Aminoacyl-tRNA synthetases have become the focus of drug discovery programs in several disease areas. − Compounds that target leucyl tRNA synthetase have already entered clinical development for TB treatment. This report focuses on lysyl tRNA synthetase (LysRS), the enzyme that charges lysyl tRNA with lysine. Aminoacyl-tRNA synthetases are an essential part of the protein biosynthesis machinery, responsible for charging tRNA with the appropriate cognate amino acid for incorporation into growing polypeptide chains. Molecules have been reported previously targeting LysRS in Plasmodium that block parasite growth. , LysS, the gene that encodes LysRS, is known to be essential for   − and has been classified in the top 200 most vulnerable genes to target for inhibition of growth. The crystal structures had confirmed that the compounds from this series were occupying the ATP pocket of LysRS.

Following the successful addition of a hydroxyl group at the two-position of the cyclohexyl ring, it was subsequently examined at the 3- and 4-positions with a methoxy at R2. At the 4-position, the hydroxyl retained potency against LysRS and gained KARS1 selectivity compared to 24. In KARS1, the equivalent residue is Asn497, which forms hydrogen bonds with the bound substrate lysine and Arg485, thereby blocking access to this part of the pocket. In LysRS, Thr425 is too distant from the bound substrate lysine and Lys413 (Arg485 in KARS1) to establish this hydrogen bond network, thereby allowing access of 27 and explaining the gain in selectivity. The crystal structure of 27 indicated that there was space to extend the hydroxy group deeper into the pocket. In a bid to develop this further, to explore the potential for interaction at the 4-position, a carbon spacer was added; again, this displayed good LysRS potency, but the slight decrease in MIC potency, for both 27 and 28, prevented further scope for optimization.

> MGSSHHHHHHSSGENLYFQGHMSAADTAEDLPEQFRIRRDKRARLLAQGRDPYPVAVPRTHTLAEVRAAHPDLPIDTATEDIVGVAGRVIFARNSGKLCFATLQDGDGTQLQVMISLDKVGQAALDAWKADVDLGDIVYVHGAVISSRRGELSVLADCWRIAAKSLRPLPVAHKEMSEESRVRQRYVDLIVRPEARAVARLRIAVVRAIRTALQRRGFLEVETPVLQTLAGGAAARPFATHSNALDIDLYLRIAPELFLKRCIVGGFDKVFELNRVFRNEGADSTHSPEFSMLETYQTYGTYDDSAVVTRELIQEVADEAIGTRQLPLPDGSVYDIDGEWATIQMYPSLSVALGEEITPQTTVDRLRGIADSLGLEKDPAIHDNRGFGHGKLIEELWERTVGKSLSAPTFVKDFPVQTTPLTRQHRSIPGVTEKWDLYLRGIELATGYSELSDPVVQRERFADQARAAAAGDDEAMVLDEDFLAALEYGMPPCTGTGMGIDRLLMSLTGLSIRETVLFPIVRPHSN> DRHHHHHHKLVPGTPP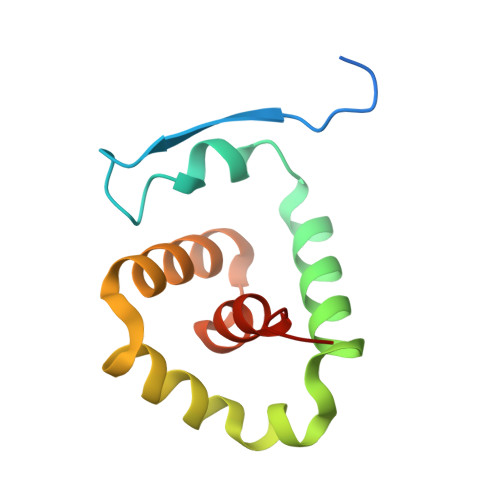LFNVSLDVAPEQRWLPMLRHYDPDFLRTAVAQVIGDRVPQWVLGMVGEIVSKVESFLPQPFTDEIRSICDSLSLSLADGILVNLAYEASAF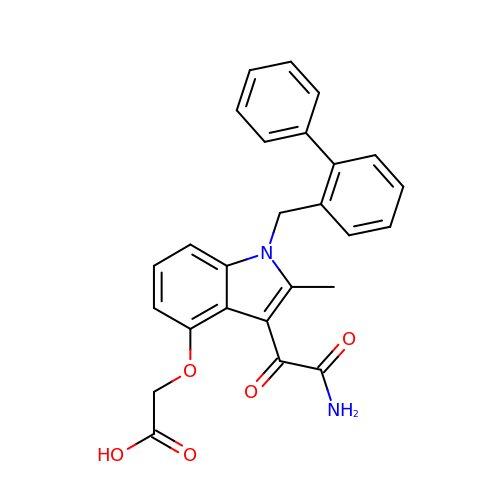2-[2-methyl-3-oxamoyl-1-[(2-phenylphenyl)methyl]indol-4-yl]oxyethanoic acid | C26 H22 N2 O5 | KFJOAXDOAYZVOY-UHFFFAOYSA-N>[5x]DYKDDDDKLHSQANLMRLKSDLFNRSPMYPGPTKDDPLTVTLGFTLQDIVKADSSTNEVDLVYWEQQRWKLNSLMWDPNEY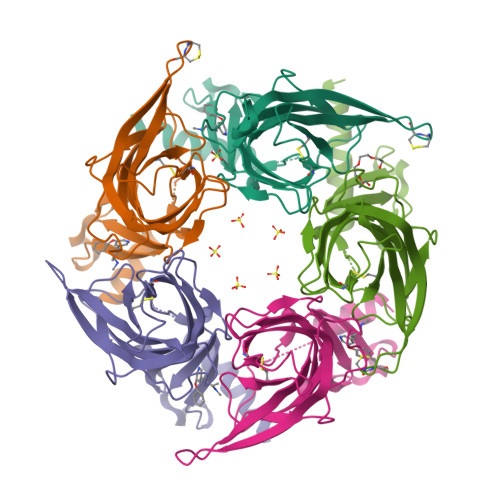GNITDFRTSAADIWTPDITAYSSTRPVQVLSPQIAVVTHDGSVMFIPAQRLSFMCDPTGVDSEEGATCAVKFGSWVYSGFEIDLKTDTDQVDLSSYYASSKYEILSATQYKHDIKYNCCEEIYPDVVLVVKFRERRAGNGFFRNLFDSR> AKMAFTLADRVTEEMLADKAALVVEVVEENYHDAPIVGIAVVNEHGRFFLRPETALADPQFVAWLGDETKKKSMFDSKRAAVALKWKGIELCGVSFDLLLAAYLLDPAQGVDDVAAAAKMKQYEAVRPDEAVYGKGAKRAVPDEPVLAEHLVRKAAAIWALERPFLDELRRNEQDRLLVELEQPLSSILAEMEFAGVKVDTKRLEQMGEELAEQLRTVEQRIYELAGQEFNINSPKQLGVILFEKLQLPVLKKTKTGYSTSADVLEKLAPYHEIVENILHYRQLGKLQSTYIEGLLKVVRPDTKKVHTIFNQALTQTGRLSSTEPNLQNIPIRLEEGRKIRQAFVPSESDWLIFAADYSQIELRVLAHIAEDDNLMEAFRRDLDIHTKTAMDIFQVSEDEVTPNMRRQAKAVNFGIVYGISDYGLAQNLNISRKEAAEFIERYFESFPGVKRYMENIVQEAKQKGYVTTLLHRRRYLPDITSRNFNVRSFAERMAMNTPIQGSAADIIKKAMIDLNARLKEERLQARLLLQVHDELILEAPKEEMERLCRLVPEVMEQAVTLRVPLKVDYHYGSTWYDAK

Recently, we investigated the mechanism of a bacterial DNA polymerase I member isolated from the thermophilic species Geobacillus stearothermophilus, Bst, by X-ray crystallography. Here we follow the reaction pathway of Bst DNA polymerase by time-resolved X-ray crystallography. In contrast to the canonical model where translocation is thought to be the last step in the catalytic cycle, time-lapsed images capturing the order and transition between intermediates demonstrate that translocation precedes phosphodiester bond formation in the mechanism of DNA synthesis. The translocation step appears to follow a push-pull mechanism where the O-O1 loop of the finger subdomain acts as a latch or pawl to facilitate unidirectional movement along the template.

For each time-dependent assay, individual crystals were transferred to an equilibration buffer [0.1 M MES (pH 7.0), 50% (NH4)2SO4, and 2.5% MPD] for 30 min at 294 K. The catalytic cycle was then initiated by transferring the crystals to reaction buffer containing 2’-deoxyadenosine triphosphate (dATP) [equilibration buffer supplemented with dATP]. The datasets acquired at 1, 4, 8, and 120 min (refined to 1.9–2.3 Å) reproducibly yield unique intermediates with high occupancy (>80%). The starting conformation observed at 0 min shows an active site configuration in which Y714 stacks directly over the 3′ end of the primer (position 10, P10) and the unpaired portion of the template strand takes a sharp turn (~90°) at the base of the finger subdomain with the next 5′ base (thymine at template position 5, T5) held outside the active site by a stacking interaction with the side chain of Y719. By 1 min, a small conformational change occurs at the base of the O-helix, leading to an opening of the O-O1 loop connecting the O and O1 helices in the finger subdomain. This movement of the finger subdomain causes the dsDNA duplex to shift ~6 Å to a position where Y714 now stacks directly over the center of the DNA duplex.> MDKKKLLYW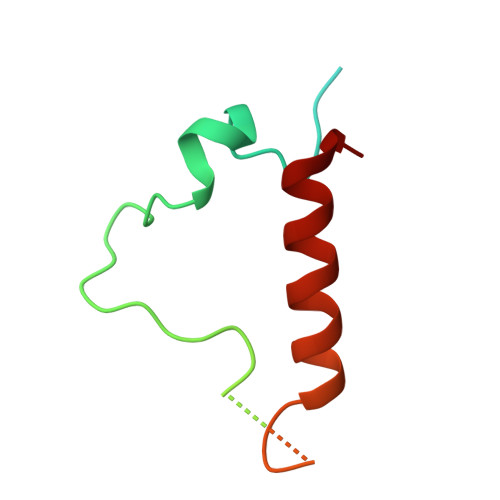VGGGLVLIIIWLWFRNRPAAQVASNWEGPPYMTYNQPQAGSVTLPVAGYTSPSLTLPNRNRSCGCNPAVSAAMAQGADLASKLTESISSQLNNYAESLNDYLASQAGV> MALR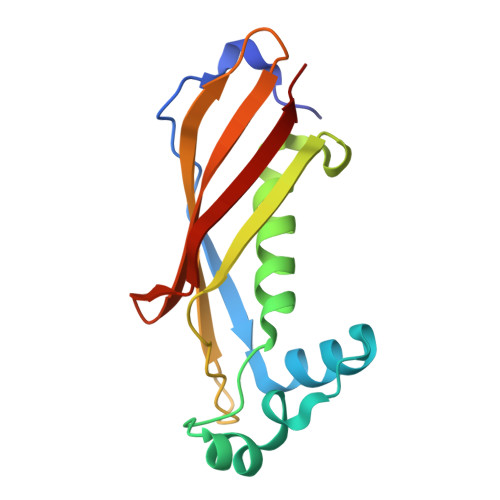EFSSVKVGDQLPEKTYPLTRQDLVNYAGVSGDLNPIHWDDEIAKVVGLDTAIAHGMLTMGIGGGYVTSWVGDPGAVTEYNVRFTAVVPVPNDGKGAELVFNGRVKSVDPESKSVTIALTATTGGKKIFGRAIASAKLA> DSEERSSWYWGRLSRQEAVALLQGQRHGVFLVRDS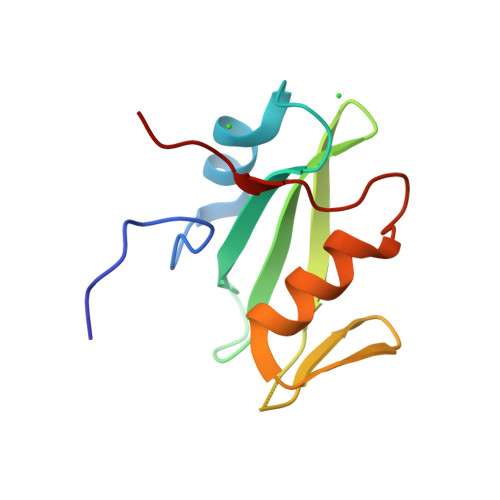STSPGDYVLSVSENSRVSHYIINSSGPRRLRIGDQEFDSLPALLEFYKIHYLDTTTLIEPVARS>QGMAKVKIVGILNVTPNSFHDGGRFVETDKAVVRARELLSQGADIIEIGGESTGPGSNTITADEELARIVPVIRAIRSSLPDANIAVDTYKAEVARKALELGATMINDVSAGRADPKLFGVVARSNAQIVLMYSKDTDPHTSFDERQYVDVVRTVYDFLAERKKAAMSAGIPADRIILDTGLGHFVSSDPQYSFQLLAHLSDFQDLGCKLFLSPSRKSFLAGNELLKTADRLPGTIAASAIAVLHGADYIRTHDVLEVRRGCEIATAINQPPER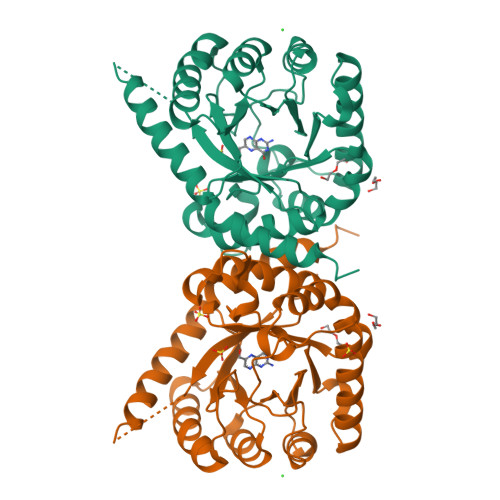[2x]>[2x]MSYKAAAGEDYKADCPPGNPAPTSNHGPDATEAEEDFVDPWTVQTSSAKGIDYDKLIVRFGSSKIDKELINRIERATGQRPHHFLRRGIFFSHR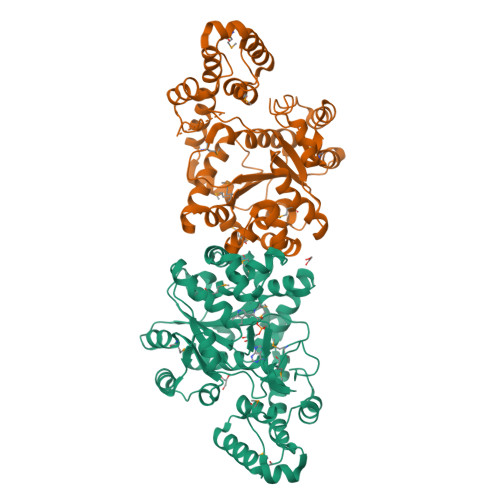DMNQVLDAYENKKPFYLYTGRGPSSEAMHVGHLIPFIFTKWLQDVFNVPLVIQMTDDEKYLWKDLTLDQAYGDAVENAKDIIACGFDINKTFIFSDLDYMGMSSGFYKNVVKIQKHVTFNQVKGIFGFTDSDCIGKISFPAIQAAPSFSNSFPQIFRDRTDIQCLIPCAIDQDPYFRMTRDVAPRIGYPKPALLHSTFFPALQGAQTKMSASDPNSSIFLTDTAKQIKTKVNKHAFSGGRDTIEEHRQFGGNCDVDVSFMYLTFFLEDDDKLEQIRKDYTSGAMLTGELKKALIEVLQPLIAEHQARRKEVTDEIVKEFMTPRKLSFDFQKLAAALEHHHHHH> KKGCVVIVGRIVLSGKPA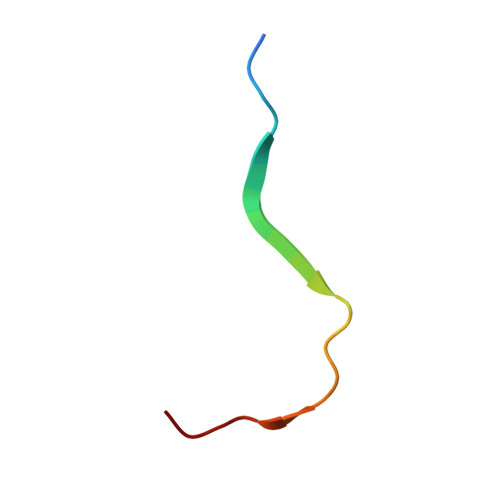IIPKK>ELPQMTQQLNSDDMQEQLSATVKFRQILSREHRPPIDVVIQAGVVPRLVEFMRENQPEMLQLEAAWALTNIASGTSAQTKVVVDADAVPLFIQLLYTGSVEVKEQAIWALGNVAGDSTDYRDYVLQCNAMEPILGLFNSNKPSLIRTATWTLSNLCRGKKPQPDWSVVSQALPTLAKLIYSMDTETLVDACWAISYLSDGPQEAIQAVIDVRIPKRLVELLSHESTLVQTPALRAVGNIVTGNDLQTQVVINAGVLPALRLLLSSPKENIKKEACWTISNITAGNTEQ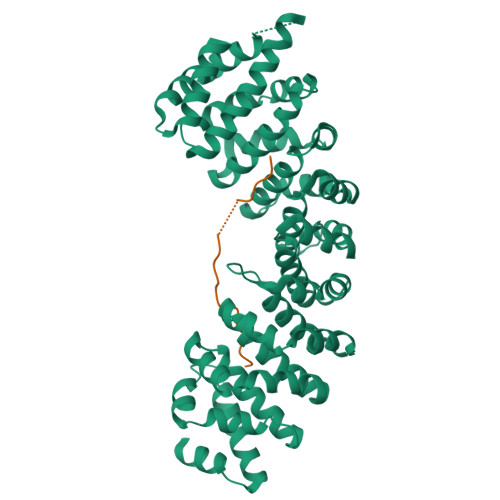IQAVIDANLIPPLVKLLEVAEYKTKKEACWAISNASSGGLQRPDIIRYLVSQGCIKPLCDLLEIADNRIIEVTLDALENILKMGEADKEARGLNINENADFIEKAGGMEKIFNCQQNENDKIYEKAYKIIETYFG[2x];>[2x]SSDTRKHKFDTSTWALPNKRRRIESEGVGTPSTSPISSLASQKSNCDSDNSITFSRDPFGWNKWKTSAIGSNSENNTSDQKNSYDRRQYGTAFIRKKKVAKQNINNTKLVSRAQSEEVTYLRQIFNGEYKVPKILKEERERQLKLMDMDKEKDTGLKKSIIDLTEKIKTILIENNKNRLQTRNENDDDLVF N~7~-(4-ethoxyphenyl)-6-methyl-N~5~-[(3S)-piperidin-3-yl]pyrazolo[1,5-a]pyrimidine-5,7-diamine | C20 H26 N6 O | 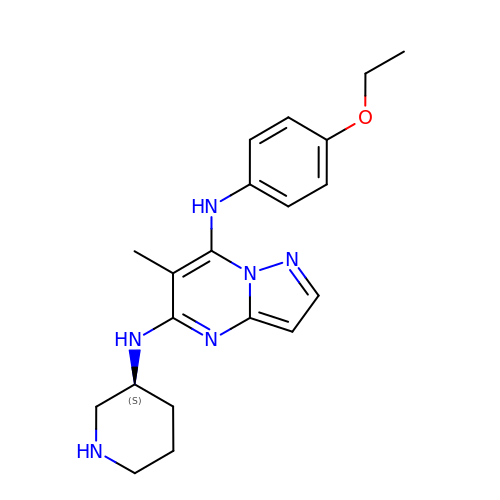WJOUGMPFYANZMI-INIZCTEOSA-N>[6x]GSHMLCAISGKVPRRPVLSPKSRTIFEKSLLEQY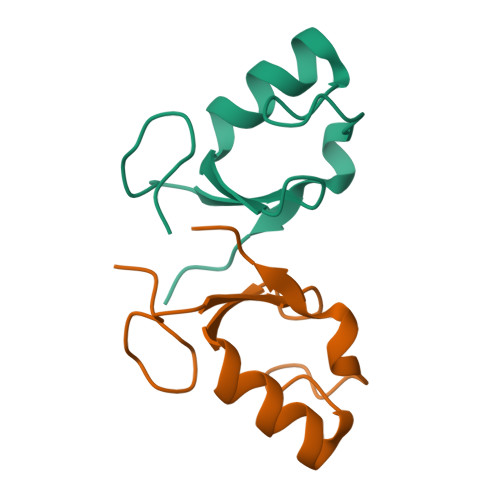VKDTGNDPITNEPLSIEEIVEIVPSAQ> MQGSVTEFLKPRLVDIEQVSSTHAKVTLEPLERGFGHTLGNALRRILLSSMPGCAVTEVEIDGVLHEYSTKEGVQEDILEILLNLKGLAVRVQGKDEVILTLNKSGIGPVTAADITHDGDVEIVKPQHVICHLTDENASISMRIKVQRGRGYVPASTRIHSEEDERPIG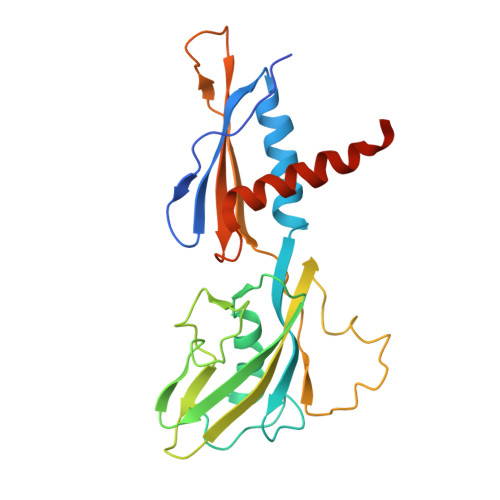RLLVDACYSPVERIAYNVEAARVEQRTDLDKLVIEMETNGTIDPEEAIRRAATILAEQLEAFVDLEVLFQ> SNAMTEESNAARPGTGASVSRRTVLAGGLAGGLALAGAPLAAAAPRGPGGPGRRDLRVMTWNIHTAVAPDAPGVVDEPRIAAVIRAEAPDVVVLNEVHRDAPGPGSHGDQPARLAELLAADGYVHTWFGLTEVDLPHEGAVLPGSSNGNVVMSRHPFVGGGVVVPLPNENYEPGGKLRRSLLTVTVDVPGLGDVVVHATHLSTPGSAVLVEDQKEQLRIVLDHVDARVPSVLAGDLNIWTTDVPTQPYSQNNLMQSWIAEDHLADTWR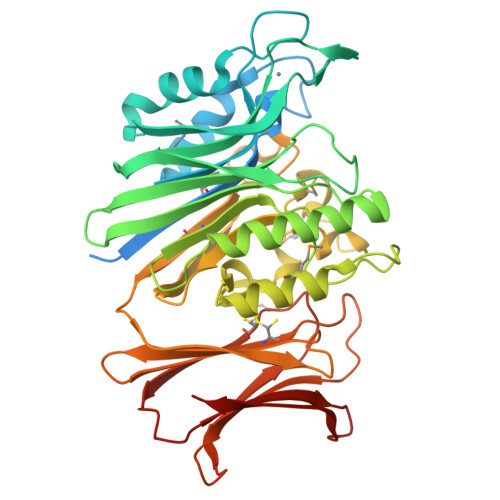QVNDPGAGPTMTASYGRPESPHPDRRIDYVFATPAFDVVAGHVSLVDRFASDHLGVVMDLRLGGAPVAARTVLAGEDGLDGWAQLTASRPGRLRLSVCKNRGQADDDGTAVRAVLRNRAGVALRTVTDSGTSRDRCTVETWRGALPPGARLEACLVGADGTILASRTETLHA> MSAVDPIADMFSAIKNAIMRRDDFLYVPSSKLKERILDVLKKEGFIQDWEALKGEKYEEEYKKMKELAEKSPNPKMKRYLK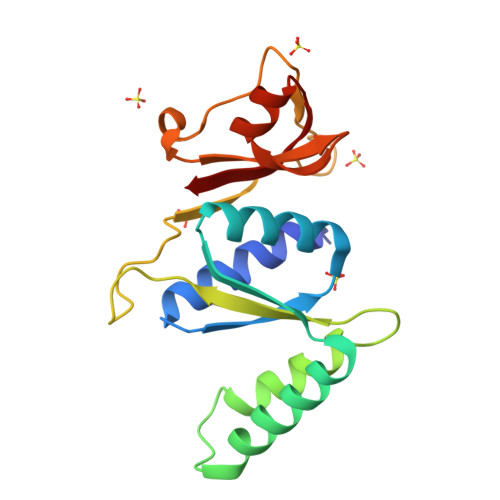QLEEYNKGTQYPIKIYLKYLDPKKRKSAITNIVKVSKGGRRVYAGVRTMPYVKRGLGIAIVSTDAGVMTDHEARRMRKGGEVIAFVW>[4x]TFLHKMGFVVTMLKLIQKKLLDKTCDQVMEFSWSALWNITDETPDNCEMFLNFNGMKLFLDCL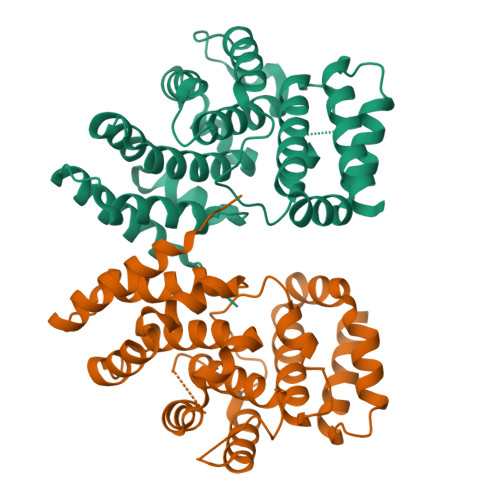KEFPEKQELHRNMLGLLGNVAEVKELRPQLMTSQFISVFSNLLESKADGIEVSYNACGVLSHIMFDGPEAWGVCEPQREEVEERMWAAIQSWDINSRRNINYRSFEPILRLLPQGISPVSQHWATWALYNLVSVYPDKYCPLLIKEGGMPLLRDIIKMATARQETKEMARKVIEHCSNFKEENMDTSR> NGPL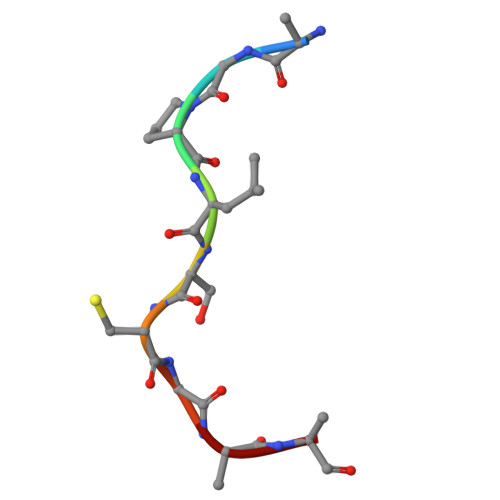SCGQR>[2x]GSAPVSIWSRVVQFGTGWGFWVSGHVFITAKHVAPPKGTEIFGRKPGDFTVTSSGDFLKYYFTSAVRPDIPAMVLENGCQEGVVASVLVKRASGEMLALAVRMGSQAAIKIGSAVVHGQTGMLLTGSNAKAQDLGTIPGDAGCPYVYKKGNTWVVIGVHVAATRSGNTVIAATHGEPTLEALEFQ

ORF2 and ORF3 encode the major and minor capsid proteins respectively, while ORF1 encodes a non-structural polyprotein that is cleaved into functional units by the viral protease (NS6pro). X-ray crystallographic analysis of the NS6 protease from three different strains of human norovirus has revealed the protein to be a cysteine protease with a chymotrypsin-like fold, similar to that of the 3C proteases from picornaviruses. The NS6pro fold is composed of two β-barrel domains tightly packed against each other; the interface between these two domains forms the peptide-binding cleft at the centre of which is the protease active site, a catalytic triad consisting of cysteine, histidine and aspartic or glutamic acid. The amino acids on the N-terminal side of the cleaved peptide bond (the P1 position in the nomenclature of Schechter and Berger) are typically glutamine or glutamic acid, while the P1′ amino acids on the C-terminal side is usually glycine or alanine; the residues at the P2 and P4 positions tend to be large and hydrophobic in nature.

To prevent autolysis of the protease in the high concentrations used for crystallisation trials MNV NS6pro was inactivated by mutation of the active site nucleophile to alanine (C139A). The protein crystallised by hanging drop vapour diffusion in 20% w/v PEG 3350, 0.2 M KSCN, 0.1 M Bis-Tris propane pH 7.5 to yield crystals that belong to space-group C2221 and have two molecules in the asymmetric unit. They diffracted X-rays to 1.6 Å resolution, producing an electron density map of extremely good quality for residues 1–123 and 132–183 in both molecules of the asymmetric unit. The active site triad of H30, D54, and C139 (A139 in our mutated protein) is located in the centre of the peptide-binding cleft formed at the interface of these two domains. Strikingly, in our structure the flexibility of the C-terminal polypeptide has actually allowed it to associate with the peptide-binding sites of a neighbouring molecule in the crystal – a happy accident that has revealed the structure of an MNV NS6pro-peptide complex. For chain A, the interaction is symmetric: it donates its C-terminus to a neighbouring A-chain that is related by crystallographic two-fold symmetry and binds the C-terminus received from this molecule. In contrast, chain B donates its C-terminus to a neighbouring B-chain but binds the C-terminus of a third molecule (also a B-chain). The adventitious insertion of the NS6pro C-terminus into the peptide-binding cleft of neighbouring proteases in our crystals has provided us with a detailed view of a structure that corresponds to the protease-product complex of MNV NS6pro that forms following cleavage of the NS6-NS7 junction in the viral polyprotein. The primary contacts with the protease are made by the carboxylate group of P1-Gln and side-chains of P1-Gln, P2-Phe and P4-Leu. P1 residue recognition by MNV NS6pro is mediated primarily by a specificity triad of residues composed of H157, T134 and Y143.>HHHHHHMTDMSEFTLKTRLLAALKGEPVDKVPVCSVTQTGIVELMDVVGAPWPEAHTNPELMAKLALANHELSGLEAVRLPYCLTVLVEAMGCEINMGTKNRQPSVTGHPYPKDLEGAAVPADLLQRGRIPVVLEAIKIIREKVGPDVPIVGGMEGPVTVASDLVSVKSFMKWSIKKTDLLEQALDIATEASIIYANAMVEAGADVIAIADPVASPDLMSPDSFRQFLKSRLQKFASSVNSVTVLHICGNVNPILSDMADCGF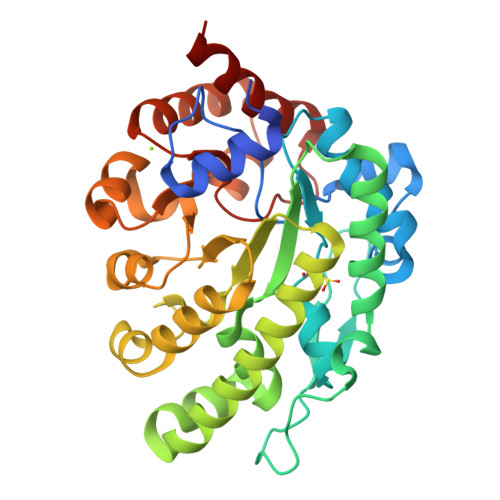EGLSVEEKIGSAKKGKEVIGTRARLVGNVSSPFTLLPGPVDKIKAEAKEALEGGIDVLAPGCGIAPMTPLENVKALVAARDEFYA[2x]> MKLAILTTLLAGASAFTTPNARPAFATKLSMSEEAAAEEAPAADAPEEVVEPASPSYTCISKEAILSSPDTTEIGRVWDPLGLA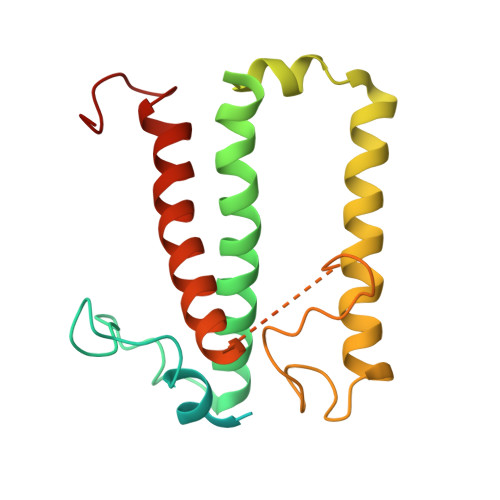EIGSAETLAWYRHSEVKHGRIAMAAFVGWWAVGAGLRFPGELSHGLEFSSIPSKGLEAWDAVPGWGKAQMLLFAGLIEFHDELFHTRRTEGGHYLRGGTPGKNMVPGLFDPFGFSKGKSEEELAKGRDREIKNGRLAMIGVAGLYCAATIPGSVPLQPPC>[2x]MPQLHYVPYDTPVEDVMRILKESGTLVIRNFLDQNTVQKVQDEVDDYVRNWNPGPKYNHDIKTVGSKTKQPSNLSLMSKTYRCEVLNHPWMHAICERMFGPTYGDYWFNGGSILHLEPGENTQPIHQDHVFYQISKWRRPTDPDLTINFTMALTEFTVENGGTRVCPGSHLWENGHASPAEEDMVPVLMQPGDALILPGSMWHSAGANRTSEYRRGFATSFHPCHFTPIESHHHLPREMVEEMTPLVQKMLGFRTLNLHNNVKVWKAGEGNLEDATGLKSVAAKLAAALEHHHHHH

Here, we report the biochemical and structural characterizations of the unusually promiscuous and catalytically versatile Fe/αKG oxygenase SptF, involved in the biosynthesis of fungal meroterpenoid emervaridones. The in vitro analysis revealed that SptF catalyzes several continuous oxidation reactions, including hydroxylation, desaturation, epoxidation, and skeletal rearrangement. Fe/αKG oxygenases utilize αKG as a co-substrate and Fe(II) as a cofactor. Through the oxidative decarboxylation of αKG, a reactive Fe(IV)-oxo intermediate is generated to activate a selective aliphatic C–H bond, which is normally difficult to cleave due to high bond-dissociation energy, and then oxidative products are generated following radical recombination.

Asn65 in SptF is uniquely substituted with threonine in the closely related AndF. To clarify the function of Asn65, we constructed the SptF N65T variant, which converted 1 into 5 as the major product, with a slight amount of 4. Notably, in the crystal structure of SptF N65T-Fe/NOG/1, a hydrogen bond was observed between the C3 ketone at the A-ring and the newly introduced Thr65. These results indicated that a subtle change of the hydrogen-bond interactions affects the position of the hydrogen atom for abstraction and determines the product specificity. As a result, N65A significantly reduced the 4 and 5 formation activity to 20% and accumulated 3, suggesting that the hydrogen-bond interaction with Asn65 is not completely essential but moderately important for the binding of 3.>[4x]MRHISPEELIALHDANISRYGGLPGMSDPGRAEAIIGRVQARVAYEEITDLFEVSATYLVATARGHISNDANKRTALNSALLFLRRNGVQ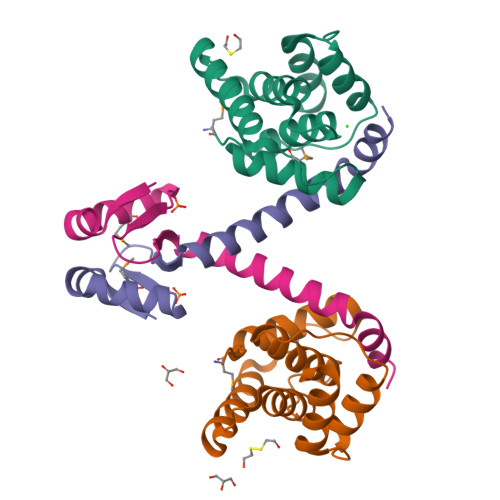VFDSPELADLTVGAATGEISVSSVADTLRRLYGSAELEHHHHHH;>[4x]MQSINFRTARGNLSEVMNNVEAGEEVEITRRGREPAVIASKATFEAYKKAALDAEFASLFDTLDSTNKELVNR> MNAKTKFDLYQHVTDRIIASIEAGTPAWRKPWTGEAATMQMPLRSNGEAYRGINVVMLWLTAAEKGYRSAY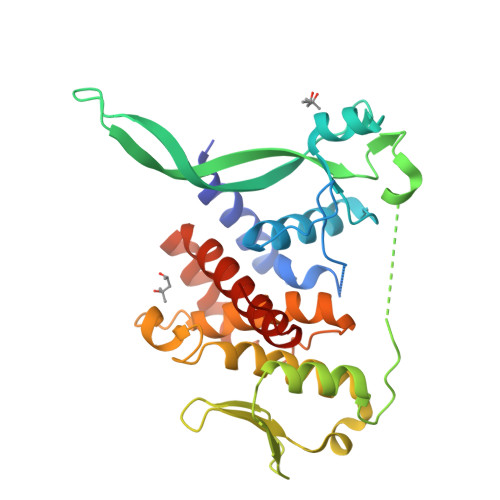WFTYRQAKELGGQVRKGEKGSTVVKFGTIEREDEQTGEEKKIPYLKGYTVFNADQIDGLPEQYHAAPAEAARDLGTAADPELDAFFAATGADIRTSSEPRAYYNPTGDYIHMPPIATFHSAAGYYATLAHEATHWTGHKSRLDRFSRFSDRKSYAFEELIAEIGNCMLCASLGLIPDFDQSAAYVQSWLRALKDDKRLIFKAATEAQKAADLLQENAANFQRKEAA>MRSDKELKFLVVDDFSTGRRIVRNLLKELGFNNVEEAEDGVDALNKLQAGGYGFVISDWNMPNMDGLELLKTIRADGAMSALPVLMVTAEAKKENIIAAAQAGASGYVVKPFTAATLEEKLNKIFEKLGM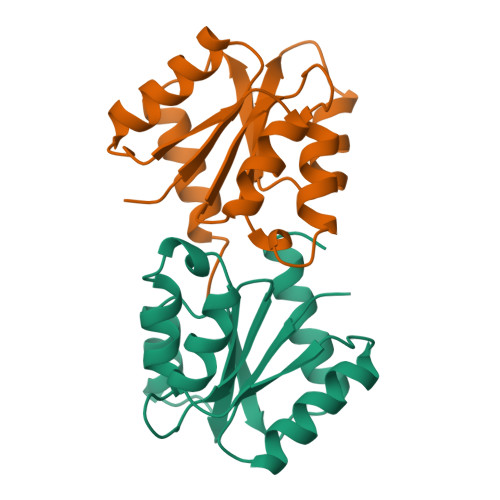[2x]> GPLGSGRMRVKAIFSHAAGDNSTLLSFKEGDLITLLVPEARDGWHYGESEKT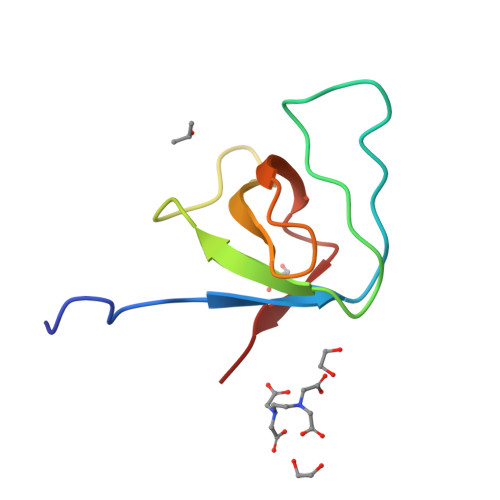KMRGWFPFSYTRVLD>SRPLSDQEKRKQISVRGLAGVENVTELKKNFNRHLHFTLVKDRNVATPRDYYFALAHTVRDHLVGRWIRTQQHYYEKDPKRIYYLSLEFYMGRTLQNTMVNLALENACDEATYQLGLDMEELEEIEEDAGLGNGGLGRLAACFLDSMATLGLAAYGYGIRYEFGIFNQKICGGWQMEEADDWLRYGNPWEKARPEFTLPVHFYGRVEHTSQGAKWVDTQVVLAMPYDTPVPGYRNNVVNTMRLWSAKAPNDFNLKDFNVGGYIQAVLDRNLAENISRVLYPNDNFFEGKELRLKQEYFVVAATLQDIIRRFKSSKFGCRDPVRTNFDAFPDKVAIQLNDTHPSLAIPELMRVLVDLERLDWDKAWEVTVKTCAYTNHTVIPEALERWPVHLLETLLPRHLQIIYEINQRFLNRVAAAFPGDVDRLRRMSLVEEGAVKRINMAHLCIAGSHAVNGVARIHSEILKKTIFKDFYELEPHKFQNKTNGITPRRWLVLCNPGLAEIIAERIGEEYISDLDQLRKLLSYVDDEAFIRDVAKVKQENKLKFAA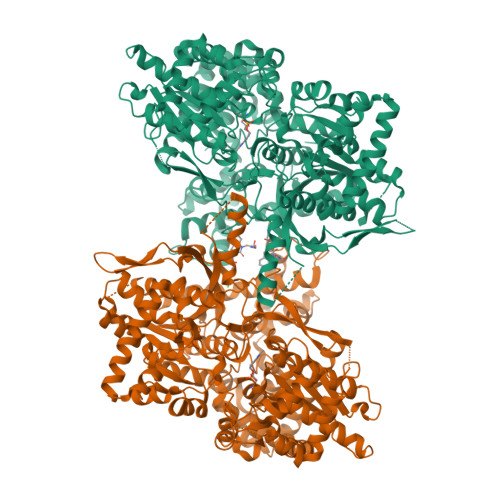YLEREYKVHINPNSLFDVQVKRIHEYKRQLLNCLHVITLYNRIKKEPNKFVVPRTVMIGGKAAPGYHMAKMIIKLITAIGDVVNHDPVVGDRLRVIFLENYRVSLAEKVIPAADLSEQISTAGTEASGTGNMKFMLNGALTIGTMDGANVEMAEEAGEENFFIFGMRVEDVDRLDQRGYNAQEYYDRIPELRQIIEQLSSGFFSPKQPDLFKDIVNMLMHHDRFKVFADYEEYVKCQERVSALYKNPREWTRMVIRNIATSGKFSSDRTIAQYAREIWGVEPSRQRLPAPDEKIP[2x]> MGGHHHHHHGENLYFQGISSETGEMGILWEFDPIINKWIRLSMKLKVERKPFAEGALREA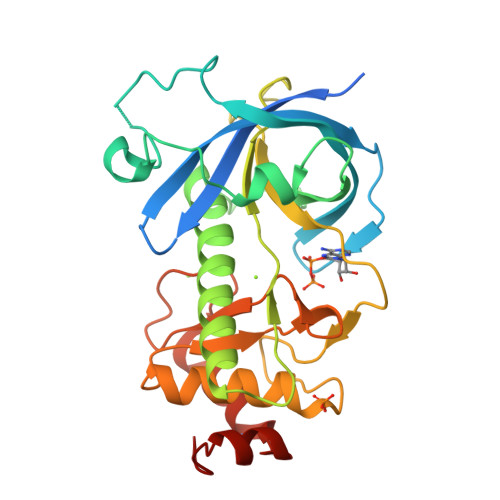YHTVSLGVGTDENYPLGTTTKLFPPIEMISPISKNNEAMTQLKNGTKFVLKLYKKEAEQQASRELYFEDVKMQMVCRDWGNKFNQKKPPKKIEFLMSWVVELIDRSPSSNGQPILCSIEPLLVGEFKKNNSNYGAVLTNRSTPQAFSHFTYELSNKQMIVVDIQGVDDLYTDPQIHTPDGKGFGLGNLGKAGINKFITTHKCNAVCALLDLDVKL Unlike the large multi-subunit complex of the proton pumping type I NADH:quinone oxidoreducatase (complex I) and the sodium pumping type NADH:quinone oxidoreducatase (NQR), the type II NADH:quinone oxidoreducatase (NDH-2) is a single subunit monotopic membrane-protein with a molecular mass range of 40–70 kDa. NDH-2 catalyses exergonic oxidation of NADH and quinone reduction through the co-factor FAD or FMN. NDH-2 comprises two Rossmann folds that are responsible for binding NADH and housing the co-factor FAD (non-covalently), are central to NADH oxidation. These domains are followed by a C-terminal membrane-anchoring domain in which the quinone-binding site (Q-site) is localised, allowing electron transfer from the reduced FAD to the acceptor quinone pooled in the membrane.

To determine the binding of HQNO to the quinone-binding site of NDH-2, we co-crystallised NDH-2 with HQNO using an improved NDH-2 crystallisation platform and determined the complex structure at 2.8 Å resolution. The structure was solved in the P21 space group with lattice parameters that were highly similar to the non-ligand bound and the NAD+-bound structures. After molecular replacement, a distinct electron density that corresponded to the HQNO quinone-head group immediately appeared at the Q-site of two NDH-2 molecules (chains B and C) in an asymmetric unit. HQNO molecules were confidently modelled in two chains. The structure shows a HQNO molecule bound in the hydrophobic Q-site localising in the C-terminal membrane-anchoring domain, which comprises three anti-parallel β-strands and the first amphipathic helix. The quinone-head group of HQNO is nested into a slot-shaped quinone-binding tunnel with only a few notable contacts established between NDH-2 and HQNO. The HQNO aromatic head group is sandwiched by a hydrophobic clamp formed by the pair of Q317 and I379 side chains, consistent with the previous MD docking model. We also noticed only one hydrogen bond, with a distance of 2.8 Å, is formed between a HQNO carbonyl oxygen and a FAD isoalloxazine N3 atom. By contrast, the HQNO alkyl carbon tail is exposed to the solvent and disordered. Our bacterial NDH-2–HQNO structure suggests the inhibition mechanism of HQNO is to block the quinone substrate accessing to the FAD isoalloxzine.

>MSKPSIVILGAGYGGIVAALGLQKRLNYNEADITLVNKNDYHYITTELHQPAAGTMHHDQARVGIKELIDEKKIKFVKDTVVAIDREQQKVTLQNGELHYDYLVVGLGSEPETFGIEGLREHAFSINSINSVRIIRQHIEYQFAKFAAEPERTDYLTIVVGGAGFTGIEFVGELADRMPELCAEYDVDPKLVRIINVEAAPTVLPGFDPALVNYAMDVLGGKGVEFKIGTPIKRCTPEGVVIEVDGEEEEIKAATVVWTGGVRGNSIVEKSGFETMRGRIKVDPYLRAPGHENIFIVGDCALIINEENNRPYPPTAQIAIQHGENVAANLAALIRGGSMTPFKPHIRGTVASLGRNDAIGIVGGRKVYGHAASWLKKLIDMRYLYLIGGLSLVLKKGRFHHHHHH[4x]> MDINGGGATLPQALYQTSGVLTAGFAQYIGVGSGNGKAAFLNNDYTKFQAGVTNKNVHWAGSDSKLSATELSTYASAKQPTWGKLIQVPSVGTSVAIPFNKSGSAAVDLSVQELCGVFSGRINTWDGISGSGRTGPIVVVYRSESSGTTELFTRFLNAKCNAETGNFAVTTTFGTSFSGGLPAGAVAATGSQGVMTALAAGDGRITYMSPDFAAPTLAGLDDATKVARVGKNVATNTQGVSPAAANVSAAIGAVPVPAAADRSNPDAWVPVFGPDNTAGVQPYPTSGYPILGFTNLIFSQCYADATQTTQVRDFFTKHYGASNNNDAAITANAFVPLPTAWKATVRASFLTASNALSIGNTNVCNGIGRPLLEA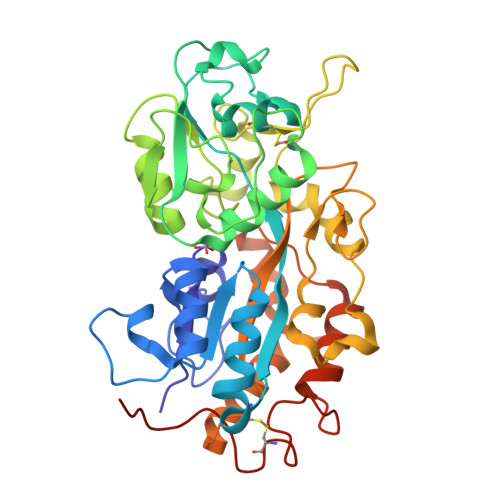AHHHHHH>GSVIDP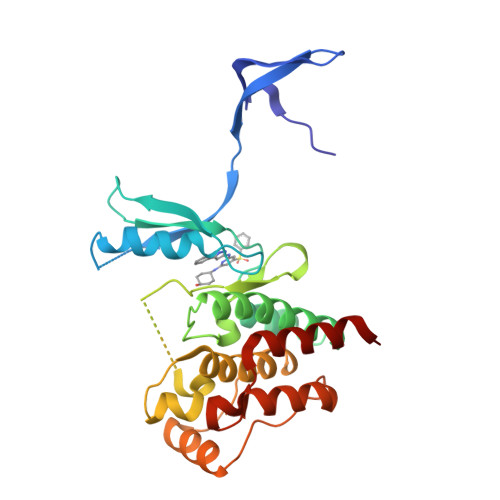SELTFVQEIGSGQFGLVHLGYWLNKDKVAIKTIREGAMSEEDFIEEAEVMMKLSHPKLVQLYGVCLEQAPICLVFEFMEHGCLSDYLRTQRGLFAAETLLGMCLDVCEGMAYLEEACVIHRDLAARNCLVGENQVIKVSDFGMTRFVLDDQETSSTGTKFPVKWASPEVFSFSRYSSKSDVWSFGVLMWEVFSEGKIPYENRSNSEVVEDISTGFRLYKPRLASTHVYQIMNHCWKERPEDRPAFSRLLRQLAEIAESGL[2x]>[6x]MTSAEMTSPNNNSEHQAIAKMRTMIEGFDDISHGGLPIGRSTLVSGTSGTGKTLFSIQFLYNGIIEFDEPGVFVTFEETPQDIIKNARSFGWDLAKLVDEGKLFILDASPDPEGQEVVGGFDLSALIERINYAIQKYRARRVSIDGVTSVFQQYDASSVVRRELF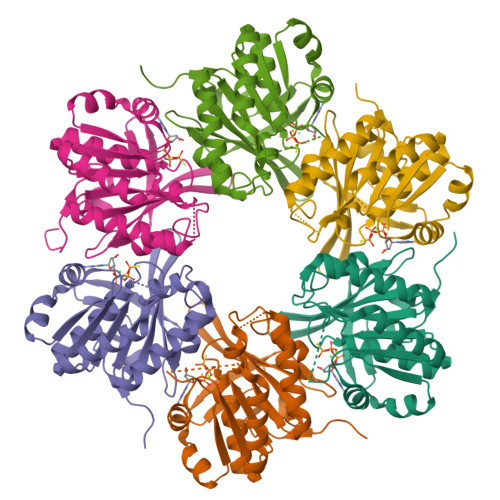RLVARLKQIGATTVMTTERIEEYGPIARYGVEEFVSDNVVILRNVLEGERRRRTLEILKLRGTSHMKGEYPFTITDHGINIFPLGAMR Growth factor signaling into mTORC1 is regulated by the heterotrimeric TSC complex, which acts as a GTPase-activating protein (GAP) for Ras homolog enriched in brain (Rheb), a GTP-binding protein that is broadly expressed in human and mammalian tissues. Rheb is a monomeric protein with a molecular weight of about 21 kDa. As in the closely related small GTPase Ras, the flexible switch I region of Rheb undergoes a conformational change during nucleotide hydrolysis and exchange, while the switch II region remains largely unchanged. Point mutations in the switch II region of Rheb (Y67A/I69A and I76A/D77A) impair its ability to activate mTORC123, implying that the switch II region is key to Rheb’s function in mTORC1 activation.

In particular, 1 showed significant chemical shift perturbations (>0.03 ppm) of 25 residues, with the most significant being Thr-61, Gly-63, Gln-64, Asp-65, Ser-75, Ile-76, Ile-78, and Val-107, all of which are present in or near the switch II domain. Further confirmation of the binding site of 1 was obtained through X-ray crystallography. 1 was then soaked into the same crystals, whereupon additional electron density was observed in the switch II domain. The 1.56 Å crystal structure of Rheb bound to 1 shows a significant ordering of the switch II loop, forming 1 turn of a helix. The dichlorophenyl moiety anchors 1 into the hydrophobic pocket of the switch II domain, while the benzimidazole nitrogens form weak interactions with the carboxylate of Glu-40 and the backbone carbonyl of Ile-69. In addition, the primary alcohol interacts with the backbone N–H of Ala-62 via a bridging water molecule. The FBLG efforts described above provided us with a small molecule Rheb binder and confirmed that the binding site was in the switch II domain. Our observations were in line with those of Maurer et al., who reported small molecule inhibitors that bind in a similar region of KRas. However, due to their weak binding affinity, we did not expect 1 or its close analogs to have functional activity. An analysis of the X-ray structure of 1 bound to Rheb showed several areas for modification with potential to gain additional interactions.

>SMPQSKSRKIAILGYRSVGKSSLTIQFVEGQFVDSYDPTIENTFTKLITVNGQEYHLQLVDTAGQDEYSIFPQTYSIDINGYILVYSVTSIKSFEVIKVIHGKLLDMVGKVQIPIMLVGNKKDLHMERVISYEEGKALAESWNAAFLESSAKENQTAVDVFRRIILEAEKLEHHHHHH[4x]>TMAGRSMQAARCPTDELSLSNCAVVSEKDYQSGQHVIVRTSPNHKYIFTLRTHPSVVPGSVAFSLPQRKWAGLSIGQEIEVALYSFDKAKQCIGTMTIEIDFLQKKNIDSNPYDTDKMAAEFIQQFNNQAFSVGQQLVFSFNDKLFGLLVKDIEAMDPSI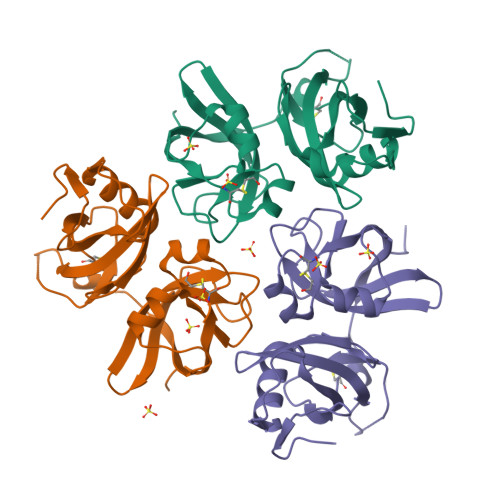LKGEPASGKRQKIEVGLVVGNSQVAFEKAENSSLNLIGKAKTKE[3x]>EPEEPTPAPWARLWALQDGFANLECVNDNYWFGRDKSCEYCFDEPLLKRTDKYRTYSKKHFRIFREVGPKNSYIAYIEDHSGNGTFVNTELVGKGKRRPLNNNSEIALSLSRNKVFVFFDLTVDDQSVYPKALRDEYIMSKTLGSGACGEVKLAFERKTCKKVAIRIISKRKFAIGSAREADPALNVETEIEILKKLNHPCIIKIKNFFDAEDYYIVLELMEGGELFDKVVGNKRLKEATCKLYFYQMLLAVQYLHENGIIHRDLKPENVLLSSQEEDCLIKITDFGHSKILGETSLMRTLCGTPTY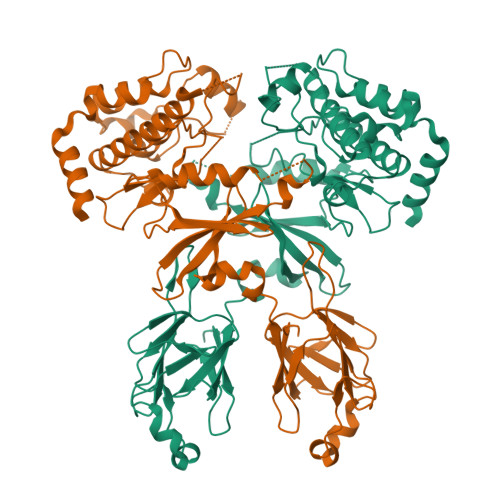LAPEVLVSVGTAGYNRAVDCWSLGVILFICLSGYPPFSEHRTQVSLKDQITSGKYNFIPEVWAEVSEKALDLVKKLLVVDPKARFTTEEALRHPWLQDEDMKRKFQDLLSEE[2x]> MSQSNRELVVDFLSYKLSQKGYSWSQFSDVEENRTEAPEGTESEMETPSAINGNPSWHLADSPAVNGATGHSSSLDAREVIPMAAVKQALREAGDEFELRYRRAFSDLTSQLHITPGT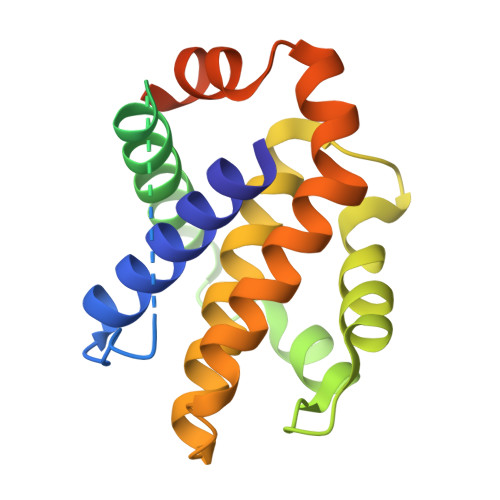AYQSFEQVVNELFRDGVNWGRIVLFFSFGGALCVESVDKEMQVLVSRIAAWMATYLNDHLEPWIQENGGWDTFVELYGNNAAAESRKGQERFNEHHHHHH> MKAIAVKRGEDRPVVIEKPRPEPESGEALVRTLRVGVDGTDHEVIAGGHGGFPEGEDHLVLGHEAVGVVVDPNDTELEEGDIVVPTVRRPPASGTNEYFERDQPDMAPDGMYFERGIVGAHGYMSEFFTSPEKYLVRIPRSQAELGFLIEPISITEKALEHAYASRSAFDWDPSSAFVLGNGSLGLLTLAMLKVDD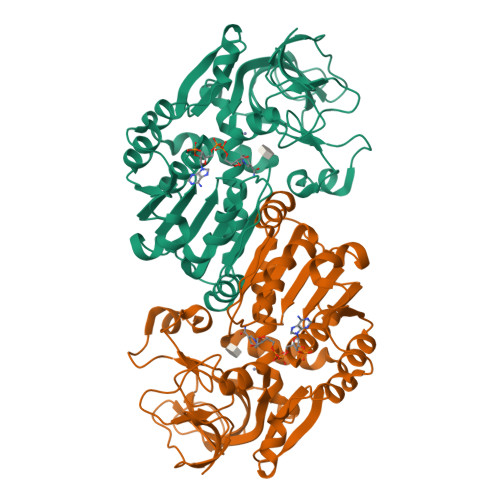KGYENLYCLGRRDRPDPTIDIIEELDATYVDSRQTPVEDVPDVYEQMDFIYEATGFPKHAIQSVQALAPNGVGALLGVPSDWAFEVDAGAFHREMVLHNKALVGSVNSHVEHFEAATVTFTKLPKWFLEDLVTGVHPLSEFEAAFDDDDTTIKTAIEFSTV> MAAGVAAWLPFARAAAIGWMPVANCPMPLAPADKNKRQDELIVLNVSGRRFQTWRTTLERYPDTLLGSTEKEFFFNEDTKEYFFDRDPEVFRCVLNFYRTGKLHYPRYECISAYDDELAFYGILPEIIGDCCYEEYKDRKRENAERLMDDNDSENNQESMPSLSFRQTMWRAFENPHTSTLALVFYYVTGFFIAVSVITNVVETVPCGTVPGSKELPCGERYSVAFFCLDTACVMIFTVEYLLRLFAAPSRYRFIRSVMSIIDVVAIMPYYIGLVMTNNEDVSGAFVTLRVFRVFRIFKFSRHSQGLRILGYTLKSCASELGFLLFSLTMAIIIFATVMFYAEKGSSASKFTSIPASFWYTIVTMTTLGYGDMVPKTIAGKIFGSICSLSGVLV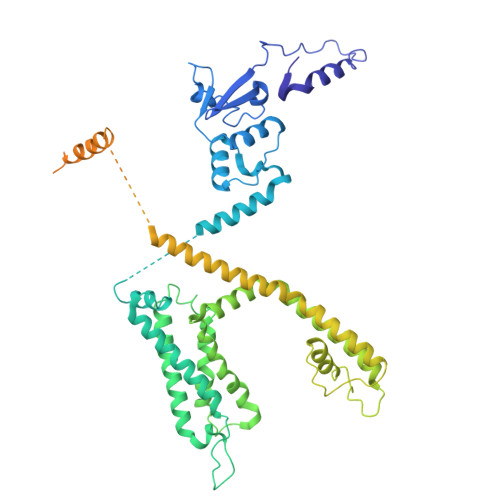IALPVPVIVSNFSRIYHQNQRADKRRAQKKARLARIRVAKTGSSNAYLHSKRNGLLNEALELTGTPEEEHMGKTTSLIESQHHHLLHCLEKTTNHEFIDEQMFEQNCMESSMQNYPSTRSPSLSSHPGLTTTCCSRRSKKTTHLPNSNLPATRLRSMQELSTIHIQGSEQPSLTTSRSSLNLKADDGLRPNCKTSQITTAIISIPTPPALTPEGESRPPPASPGPNTNIPSIASNVVKVSAL> MHHHHHHSSLCKTRLQEERKQWRRDHPFGFYAKPCKSSDGGLDLMNWKVGIPGKPKTSWEGGLYKLTMAFPEEYPTRPPKCRFTPPLFHPNVYPSGTVCLSILNEEEGWKPAITIKQILLGIQDLLDDPNIASPAQTEAYTMFKKDKVEYEKRVRAQAREN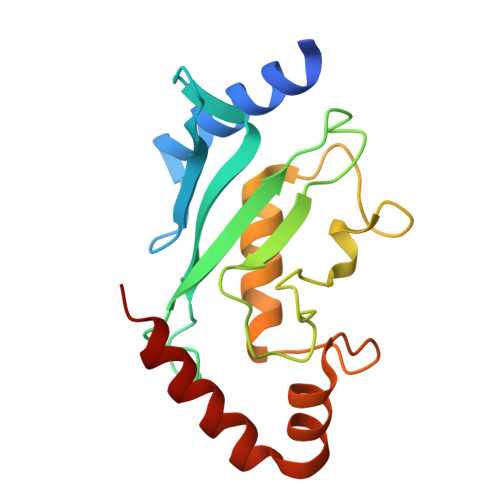AP4-ethoxyquinazoline 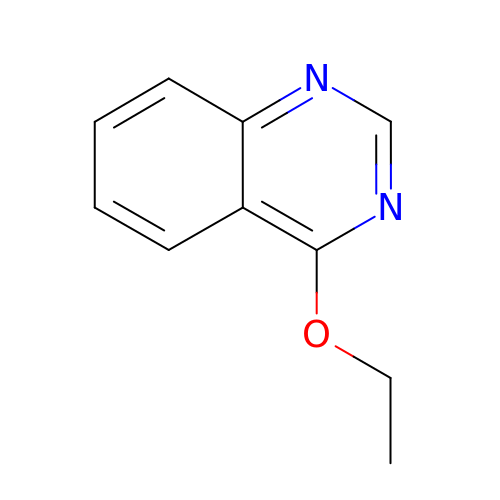| C10 H10 N2 O | KHYIWRGNPLBXDS-UHFFFAOYSA-N~{N}-[3-acetamido-5-[(3-methylcinnolin-5-yl)carbamoyl]phenyl]furan-2-carboxamide | C23 H19 N5 O4 | 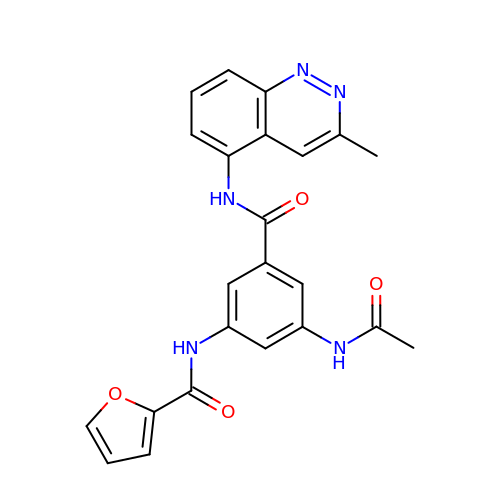KNUFZYGMIQUYJP-UHFFFAOYSA-N>[2x]LDNGLLQTPPMGWLAWERFRCNINCDEDPKNCISEQLFMEMADRMAQDGWRDMGYTYLNIDDCWIGGRDASGRLMPDPKRFPHGIPFLADYVHSLGLKLGIYADMGNFTCMGYPGTTLDKVVQDAQTFAEWKVDMLKLDGCFSTPEERAQGYPKMAAALNATGRPIAFSCSWPAYEGGLPPRVQYSLLADICNLWRNYDDIQDSWWSVLSILNWF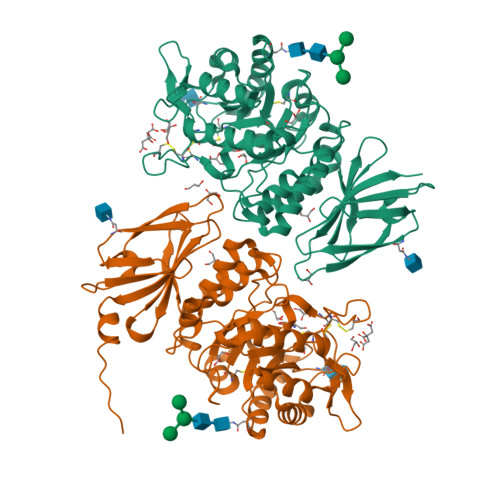VEHQDILQPVAGPGHWNDPDMLLIGNFGLSLEQSRAQMALWTVLAAPLLMSTDLRTISAQNMDILQNPLMIKINQDPLGIQGRRIHKEKSLIEVYMRPLSNKASALVFFSCRTDMPYRYHSSLGQLNFTGSVIYEAQDVYSGDIISGLRDETNFTVIINPSGVVMWYLYPIKNLEMSQQHHHHHH7-HYDROXY-5-METHYL-3,3A,5,11B-TETRAHYDRO-1,4-DIOXA-CYCLOPENTA[A]ANTHRACENE-2,6,11-TRIONE 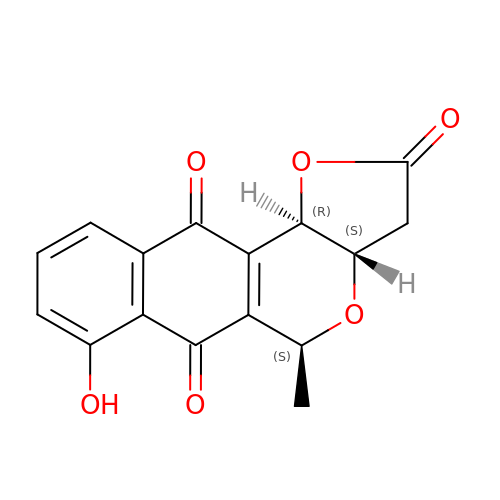| C16 H12 O6 | XUWPJKDMEZSVTP-UOSCCXBLSA-N1-bromanyl-4-methyl-benzene | C7 H7 Br | 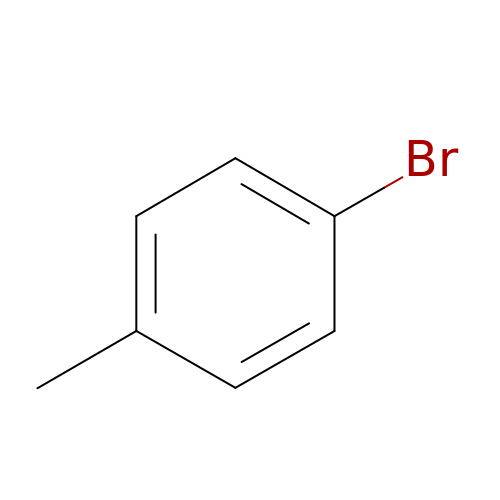ZBTMRBYMKUEVEU-UHFFFAOYSA-N>[6x]GSPPGTVDKKMVEKCWKLMDKVVRLCQNPKLALKNSPPYILDLLPDTYQHLRTILSRYEGKMETLGENEYFRVFMENLMKKTKQTISLFKEGKERMYEENSQPRRNLTKLSLIFSHMLAELKGIFPSGLFQGDTFRITKADAAEFWRK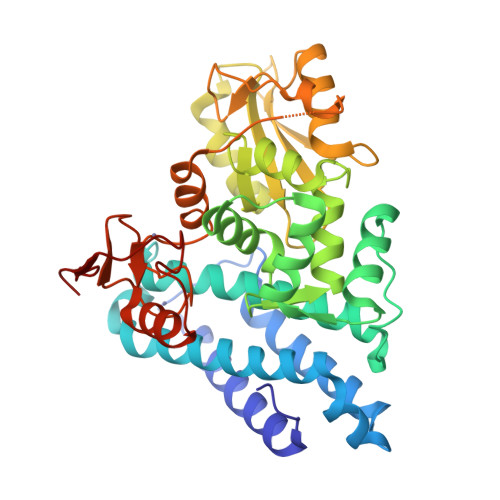AFGEKTIVPWKSFRQALHEVHPISSGLEAMALKSTIDLTCNDYISVFEFDIFTRLFQPWSSLLRNWNSLAVTHPGYMAFLTYDEVKARLQKFIHKPGSYIFRLSCTRLGQWAIGYVTADGNILQTIPHNKPLFQALIDGFREGFYLFPDGRNQNPDLTGLCEPTPQDHIKVTQEQYELFCEMGSTFQLCKICAENDKDVKIEPCGHLMCTSCLTSWQESEGQGCPFCRCEIKGTEPIVVDPFD3-phenyl-5-(1H-pyrazol-3-yl)isoxazole 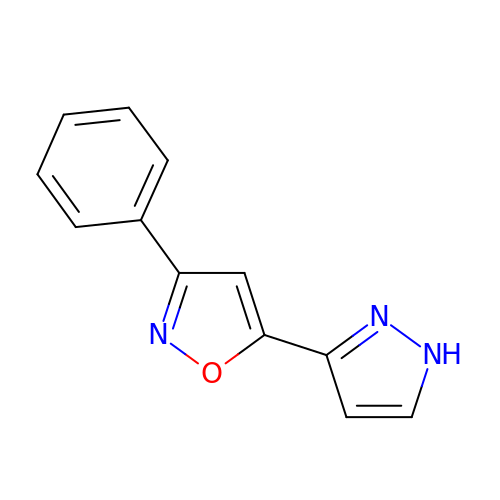| C12 H9 N3 O | SRSSTOPJERVMRZ-UHFFFAOYSA-N> GFNYDEAQVPKYTLPDPLVMVDGTKVTSAKQWNDKRRDEVQQLFEAYMYGKVPDGETELIFTDAKGERALGGAAIRKQVKISFGEKEDAPAMDLLIYLPADAKVRVPVFLGLNFHGNHTIHKDKEIWLTESWVRTNKKFGITKNKANELSRGVAAGRWQIEKAIAKGYGVATIYCGDIDPDFNFPSNGIQAYYYKKDQTIPEKGQWGTIAAWAFGLSCAMDYFETDTDIDHKKVAVLGHSRLGKTSLWAGAIDTRFALTISNCSGCGGAALSRRRFGETVRRINTSFPHWFCSRFHQYNDKEDKLPIDQHMLIALCAPRPVLINSATEDKWADPHGEFLAAQGADAVYRMLGTGGLDAKKWPEPNKLVKSTIGYHLRPGKHDVTARDWDVYIEFADHHM

The CAZymes family 15 carbohydrate esterases (CE15s) include members with glucuronoyl esterase activity that are predicted to act on the ester linkages between the 4-O-methyl-glucuronoyl substitutions on xylan of hemicellulose and the aromatic alcohol of lignin as their natural substrate; the so-called lignin-carbohydrate-complex (LCC). To discover the real conformation of these non-homologous regions, as well as determine the catalytic site residues, we have solved the crystal structure of MZ0003 to 1.9 Å. This represents the first structure of a bacterial CE15 enzyme, and is the third and most divergent CE15 structure reported. In summary, the deeper, positively charged substrate binding pocket which is formed by a novel sub-domain in MZ0003 is likely responsible for its broader substrate specificity relative to fungal homologs, and indicates diversity of activity may exist among unexplored clades of CE15 enzymes.

The overall topology of MZ0003 reveals the presence of three large inserts, referred to as regions 1, 2 and 3, which do not have counterparts in either of the fungal homologs. Region 2 is a 45 residue loop between β5 and β6 which includes three 310 helices and a short (6 residue) α-helix (α6). Together, regions 1 and 2 form a subdomain at the N-terminal end of the central β-sheet, with the helices of region 2 on the same side as the catalytic residues and the loops of region 2 protruding over the active site and partially occluding it. In addition to narrowing the access to the active site, region 2 includes several basic residues, namely Arg 137, Asn 139, Lys 140 and 141, Arg 160, which contribute to the positively charged surface potential surrounding the catalytic pocket. The relatively occluded access to the catalytic residues, suggests that MZ0003 may act on smaller or fragmented substrates rather than the intact LCC polymers that are the proposed target of the fungal enzymes. The geometric arrangement in the active site indicates that Asp 332 is the third residue of the triad in MZ0003, functioning to adjust the basic character of His 343. This was confirmed as the Asp332Ala mutant of MZ0003 is inactive in assays with both p-nitrophenyl acetate (p-NP acetate) and methyl 4-O-methyl-D-glucopyranuronate (data not shown). Electron density found in the active site, is consistent with a molecule of glycerol and interacts with the catalytic Ser 243 OD (2.78 Å), the side chain of Glu 281 (bidentate interactions O2 – OE1 of 2.42 Å and O3 – OE2 of 2.56 Å) and Lys 247 (2.70 Å). None of the six cysteine residues of MZ0003, which are all found in the conserved core regions of the protein, are involved in disulphide bonds in the crystal structure. The loop/helix region consisting of residues 187–206 extends from one monomer forming a “hook” which is embedded in the second molecule of the MZ0003 dimer.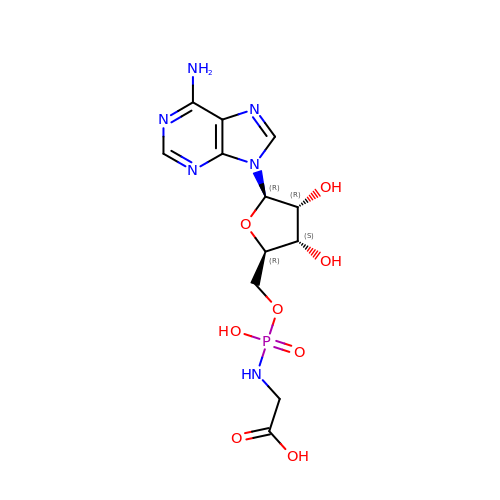2-[[[(2~{R},3~{S},4~{R},5~{R})-5-(6-aminopurin-9-yl)-3,4-bis(oxidanyl)oxolan-2-yl]methoxy-oxidanyl-phosphoryl]amino]ethanoic acid | C12 H17 N6 O8 P | OFENVOUOJQRLCP-JJNLEZRASA-N> GSHMDNQCTVQVRLELGHRAQLRKKPTTEGFTHDWMVFVRGPEQCDIQHFVEKVVFWLHDSFPKPRRVCKEPPYKVEESGYAGF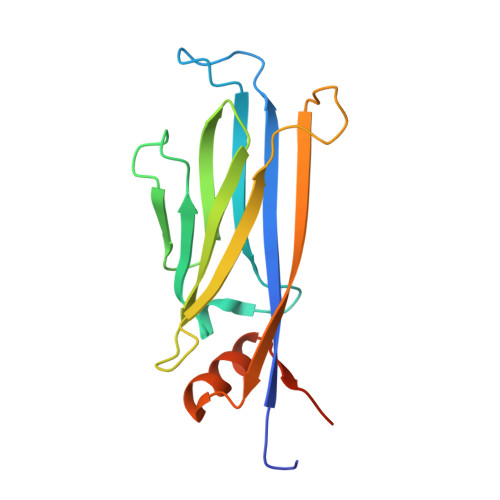IMPIEVHFKNKEEPRKVCFTYDLFLNLEGNPPVNHLNHLRCEKLTFNNPTTEFRYKLLRAGGVMVMPEGAHHHHHH> MGHHHHHHMVRVAINGFGRIGRLVMRIALSRPNVEVVALNDPFITNDYAAYMFKYDSTHGRYAGEVSHDDKHIIVDGKKIATYQERDPANLPWGSSNVDIAIDSTGVFKELDTAQKHIDAGAKKVVITAPSSTAPMFVMGVNEEKYTSDLKIVSNASCTTNCLAPLAKVINDAFGIEEGLMTTVHSLTATQKTVDGPSHKDWRGGRTASGNIIPSSTGAAKAVGKVLPELQGKLTGMAFRVPTVDVSVVDLTVKLNKETTYDEIKKVVKAAAEGKLKGVLGYTEDAVVSSDFLGDSHSSIFDASAGIQLSPKFVKLVSWYDNEYGYS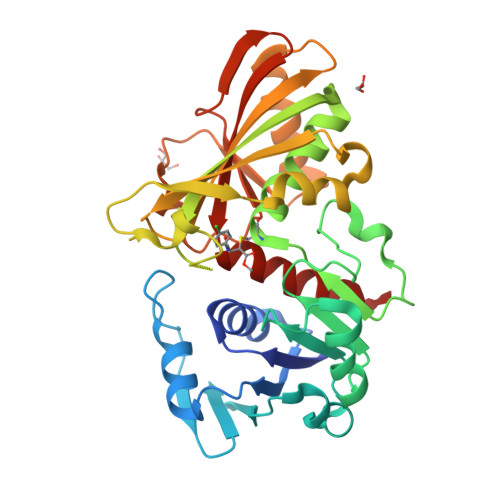TRVVDLVEHVAKA>MGIMAASRPLSRFWEWGKNIVCVGRNYADHVREMRSAVLSEPVLFLKPSTAYAPEGSPILMPAYTRNLHHELELGVVMGKRCRAVPEAAAMDYVGGYALCLDMTARDVQDECKKKGLPWTLAKSFTASCPVSA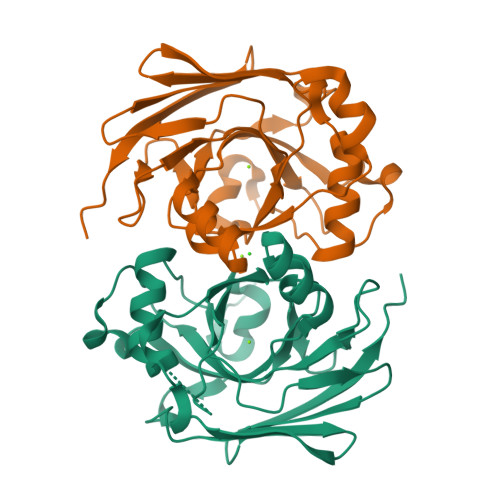FVPKEKIPDPHKLKLWLKVNGELRQEGETSSMIFSIPYIISYVSKIITLEEGDIILTGTPKGVGPVKENDEIEAGIHGLVSMTFKVEKPEY[2x]5-[2,6-di(morpholin-4-yl)pyrimidin-4-yl]-4-(trifluoromethyl)pyridin-2-amine 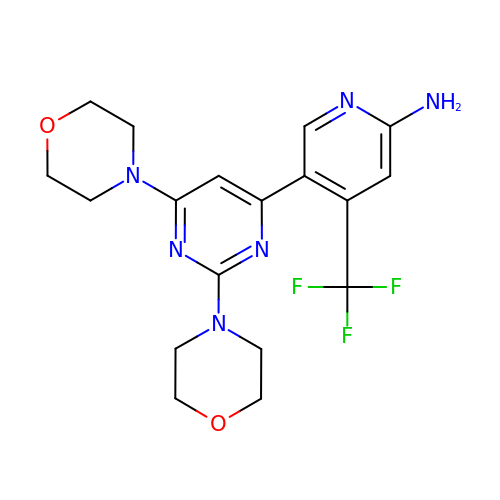| C18 H21 F3 N6 O2 | CWHUFRVAEUJCEF-UHFFFAOYSA-N> ELVLALYDYQEKSPREVTMKKGDILTLLNSTNKDWWKVEVNDRQGFVPAAYVKKLD

In this work, we report the first SSX experiments with viscous jets conducted at ALBA beamline BL13-XALOC. Small crystals (15–30 µm) of five soluble proteins (lysozyme, proteinase K, phycocyanin, insulin and α-spectrin-SH3 domain) were suspended in lipidic cubic phase (LCP) and delivered to the X-ray beam with a high-viscosity injector developed at Arizona State University. Complete data sets were collected from all proteins and their high-resolution structures determined. The high quality of the diffraction data collected from all five samples, and the lack of specific radiation damage in the structures obtained in this study, confirm that the current capabilities at the beamline enables atomic resolution determination of protein structures from microcrystals as small as 15 µm using viscous jets at room tem­per­ature.

In addition to the standard model system, i.e. proteins such as hen egg-white lysozyme and proteinase K from Tritirachium album limber, we included phycocyanin from Thermosynechococcus elongatus, human insulin and the SH3 domain of α-spectrin (α-spectrin-SH3) from Gallus gallus.>[2x]SAEKLFTPLKVGAVTAPNRVFMAPLTRLRSIEPGDIPTPLMGEYYRQRASAGLIISEATQISAQAKGYAGAPGLHSPEQIAAWKKITAGVHAEDGRIAVQLWHTGRISHSSIQPGGQAPVSASALNANTRTSLRDENGNAIRVDTTTPRALELDEIPGIVNDFRQAV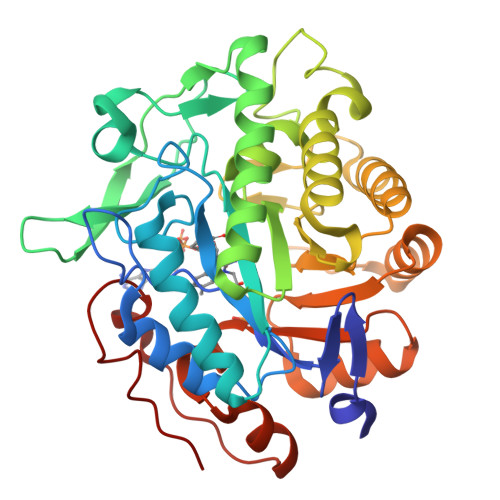ANAREAGFDLVELHSAHGYLLHQFLSPSSNQRTDQYGGSVENRARLVLEVVDAVCNEWSADRIGIRVSPIGTFQNVDNGPNEEADALYLIEELAKRGIAYLHMSETDLAGGKPYSEAFRQKVRERFHGVIIGAGAYTAEKAEDLIGKGLIDAVAFGRDYIANPDLVARLQKKAELNPQRPESFYGGGAEGYTDYPSL> MADEERLKEFKEANKIVFDPNTRQVWENQNRDGTKPATTFQSEEDIKRAAPESEKDTSATSGIVPTLQNIVATVTLGCRLDLKTVALHARNAEYNPKRFAAVIMRIREPKTTALIFASGKMVVTGAKSEDDSKLASRKYARIIQKIGFAAKFTDFKIQNIVGSCDVKFP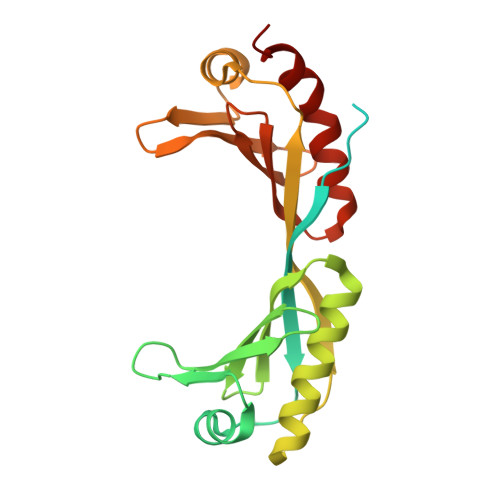IRLEGLAFSHGTFSSYEPELFPGLIYRMVKPKIVLLIFVSGKIVLTGAKQREEIYQAFEAIYPVLSEFRKM Lysins are lytic proteins that locally degrade the cell wall, either to provide access to the inner bacterial membrane during infection or to release virus progeny by cell lysis. P5ΔV8 adopts a lysozyme superfamily fold consisting of an N-terminal lobe (NTL) and a C-terminal lobe (CTL) connected by a central helix. The two lobes create a substrate binding cleft containing the predicted catalytic residue Glu95. However, in LTs, there is only one acidic residue, typically a glutamic acid, in the vicinity of the substrate cleavage site. Φ6 P5 adopts a lysozyme superfamily fold and our structure of P5 bound to a tetrasaccharide substrate analog shows that the enzyme contains a single glutamate (Glu95) in its active site. Together, our structural data unambiguously identify Φ6 P5 as an LT.

The G2238T mutation corresponds to a V207F amino-acid substitution in the gene for the lysin protein P5, which locally degrades the cell wall, either to provide access to the inner bacterial membrane during infection or to release virus progeny by cell lysis. To understand the molecular basis of the thermostabilization of P5 by the V207F mutation we determined the crystal structures of P5ΔV8wt and P5ΔV8V207F at 1.4 Å resolution (we could not obtain crystals of P5wt or P5V207F). The structures of P5ΔV8wt and P5ΔV8V207F are almost identical, with a root mean square deviation (rmsd) of the Cα positions of 0.135 Å. Residue 207 is located on helix α8, facing the hydrophobic core of the protein. The larger phenylalanine side chain in P5ΔV8V207F neatly fills the cavity, with no significant changes in the protein. The only significant side chain shift observed in P5ΔV8V207F is an adjustment in the N179 side chain to accommodate the F207 side chain, resulting in a van der Waals interaction between these two side chains. By filling an unoccupied hydrophobic cavity, the V207F substitution increases the buried hydrophobic surface area in the protein. This provides a likely explanation for the increased thermostability of the mutant, because the hydrophobic surface area that is buried within a folded protein contributes directly to its free energy of stabilization. Similarly, the melting temperatures of P5wt and P5V207F determined by DSC were 52.6°C and 58.3°C, respectively. These data indicate that the V207F mutation increases the melting temperature of P5 by between 5.7–7.6°C. Additionally, the heights and areas of the DSC curves were greater for the V207F mutants than for their wildtype counterparts. The V207F mutation did not affect the structure of the P5 active site, allowing the mutant enzyme to fully maintain its functional role as a lysin, which is essential in the viral lifecycle.

>LQALLPKAQSVGNSRVRFTTAEVDSAVARISQKIGVPASYYQFLIPIENFVVAGGFETTVSGSFRGLGQFNRQTWDGLRRLGRNLPAFEEGSAQLNASLYAIGFLYLENKRAYEASFKGRVFTHEIAYLYHNQGAPAAEQYLTSGRLVYPKQSEAAVAAFAAARNQHVKESWA[2x]> MASVPENQAPKAIFTFSPEDPVTDENVVFNASNSIDEDGTIAYYVWDFGDGYEGTSTTPTITYKYKNPGTYKVKLIVTDNQGASSSFTATIKVTSAT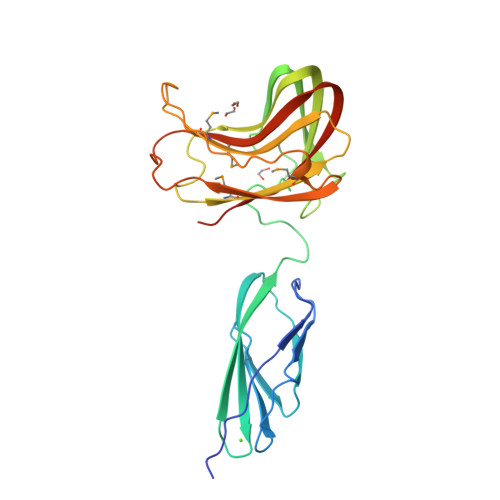GDNSKFNFEDGTLGGFTTSGTNATGVVVNTTEKAFKGERGLKWTVTSEGEGTAELKLDGGTIVVPGTTMTFRIWIPSGAPIAAIQPYIMPHTPDWSEVLWNSTWKGYTMVKTDDWNEITLTLPEDVDPTWPQQMGIQVQTIDEGEFTIYVDAIDWLEHHHHHH>ATTITSNQTGTHDGYDYELWKDSGNTSMTLNSGGAFSAQWSNIGNALFRKGKKFDSTKTHSQLGNISINYNATFNPGGNSYLCVYGWTKDPLTEYYIVDNWGTYRPTGTPKGTFTVDGGTYDIYETTRINQPSIIGIATFKQYWSVRQTKRTSGTVSVSEHFKKWESLGMPMGKM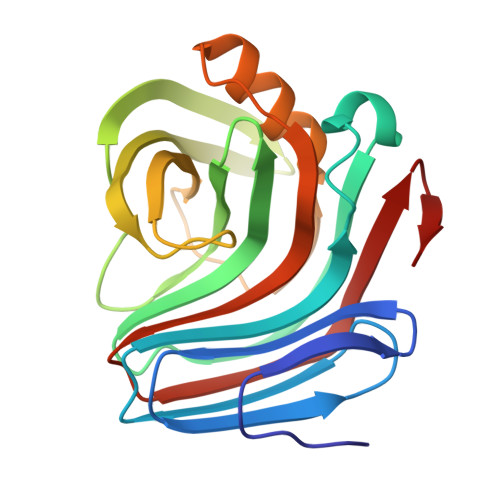YETALTVEGYQSNGSANVTANVLTIGGKPL[2x]> MFSRGAAATAMAKVSRLVSPRLRIIHRDYLTRRGGRTHQRCSAVAVDYTPTYFATYKSDPGQCPRLIDAEAVHGDEQAFWSARRDFYRGGASRSYYPAWDRQAQALIMLTREVPRIPQEAAFRLFTLGLKMMLLPRLVAGVELMLPSWVTMNAESVLNEGLEGKVAEADGDGKATGAAADAAALPSASSAGANE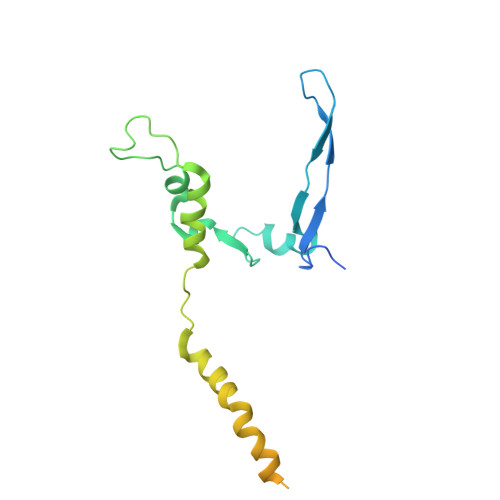DSGSANAEKR> ASMTGGQQMGRGSEFMGQSHTHDHHHDGYQAPPEDIALRVKALESLLIEKGLVDPAAMDLVVQTYEHKVGPRNGAKVVAKAWVDPAYKARLLADGTAGIAELGFSGVQGEDMVILENTPAVHNVFVCTLCSCYPWPTLGLPPAW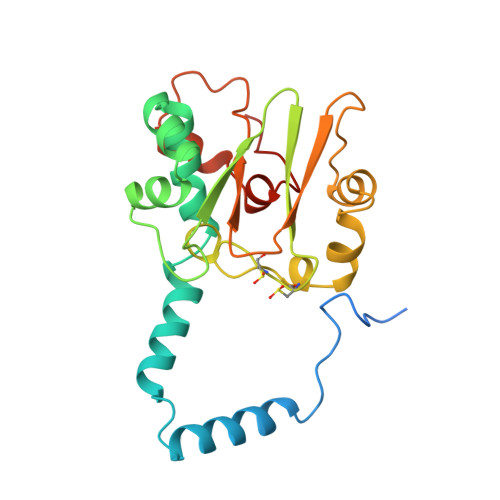YKAAPYRSRMVSDPRGVLAEFGLVIPANKEIRVWDTTAELRYMVLPERPAGTEAYSEEQLAELVTRDSMIGTGLPTQPTPSH> GGEVRQVSKHAFSLKQLDNPARIPPCGWKCSKCDMRENLWLNLTDG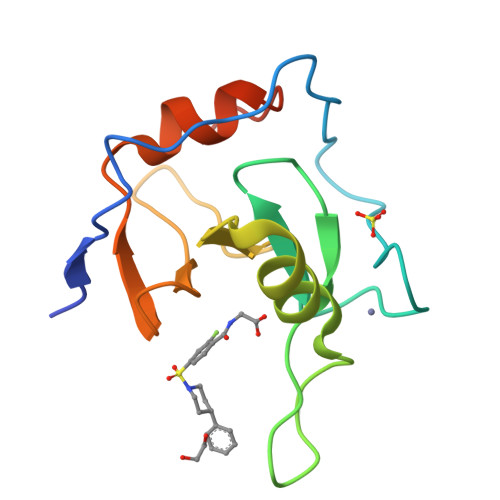SILCGRRYFDGSGGNNHAVEHYRETGYPLAVKLGTITPDGADVYSYDEDDMVLDPSLAEHLSHFGIDMLKMQKTD> AMFLQRPKPYSDESLESFFIRVANKNGYGDVHRFLEATKRFLQDIDHNGYQTFPTDITRINPYSAKNSSSARTASFLKLAQLTFNEPPELLGLAINRTNMKYSPSTSAVVRGAEVFPRSLLRTHSIPCCPLCLRENGYASYLWH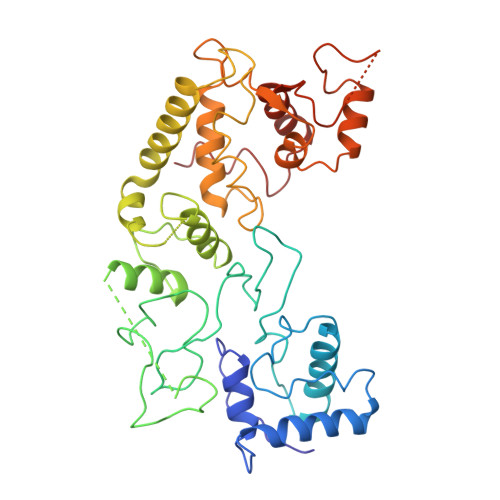FQGYEYCHSHNVPLITTCSGHEAACTVSNWLAGHESKPLPNLPKSYRWGLVHWWMGIKDSDHFSFVQFFSNWPRSFHSIIEDEVEFNLEHAVVSTSELRLKDLLGRLFFGSIRLPERNLQHNIILGELLCYLENRLWQDKGLIANLKMNALEATVMLNCSLDQIASMVEQRILKPNRKSKDVTDYLFHFGDIFCLWLAEFQSDEFNRSFYVSRW> MEFTVSTTEDLQRYRTECVSSLNIPADYVEKFKKWEFPEDDTTMC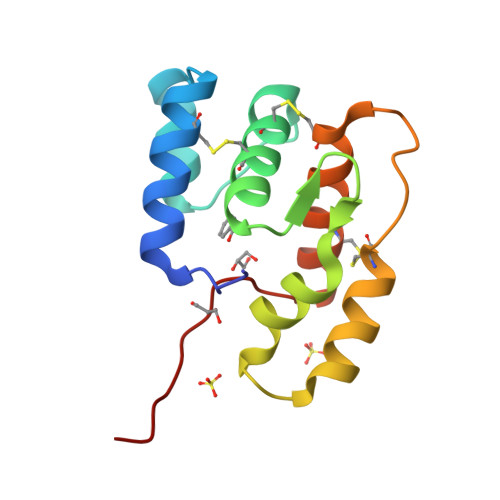YIKCVFNKMQLFDDTEGPLVDNLVHQLAHGRDAEEVRTEVLKCVDKNTDNNACHWAFRGFKCFQKNNLSLIKASIKKD>[8x]MSQSVSERTRIKSDRYESGVIPYAKMGYWDAAYTVKDTDVLALFRITPQPGVDPVEAAAAVAGESSTATWTVVWTDLLTACERYRAKAYRVDPVPNSTDVYFAFIAYECDLFEEASLANLTASIIGNVFGFKAISALRLEDMRIPHSYLXTFQGPATGIIVERERLNKYGTPLLGATVKPKLGLSGKNYGRVVYEGLKGGLDFLKDDENINSQPFMRWRERFLNCLEGINRASAATGEVKGSYLNVTAATMEEVYKRAEYAKAIGSIVVMIDLVMGYTAIQSIAYWARENDMLLHLHRAGNSTYARQKNHGINFRVICKWMRMSGVDHIHAGTVVGKLEGDPLMIKGFYDILRLTELEVNLPFGIFFEMDWASLRRCMPVA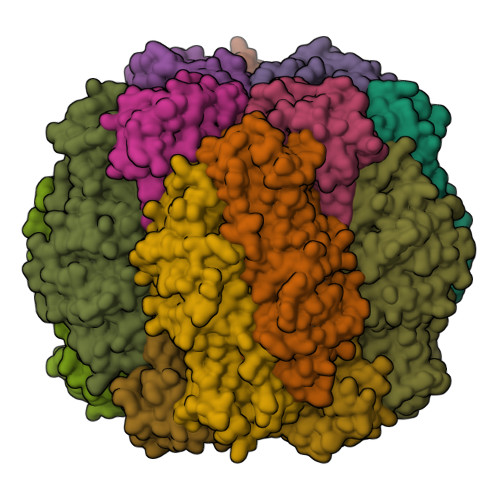SGGIHCGQMHQLIHYLGDDVVLQFGGGTIGHPDGIQAGATANRVALEAMVLARNEGADYFNNQVGPQILRDAAKTCGPLQTALDLWKDISFNYTSTDTADFSETATANR;>MRLTQGCFSFLPDLTDAQIEKQVAYAMSRGWAMNVEWTDDPHPRNNYWELWGLPLFDIKDPATVMFELNEARKSCAAGYIRMNAFDASYGTESCVMSFLTNRPANEPGFYLDRTDGIGRQIIYSIKSYSVQANPEGSRY[8x]> MVALSLKISIGNVVKTMQFEPSTMVYDACRMIRERIPEALAGPPNDFGLFLSDDDPKKGIWLEAGKALDYYMLRNGDTMEYRKKQRPLKIRMLDGTVKTIMVDDSKTVTDMLMTICARIGITNHDEYSLVRE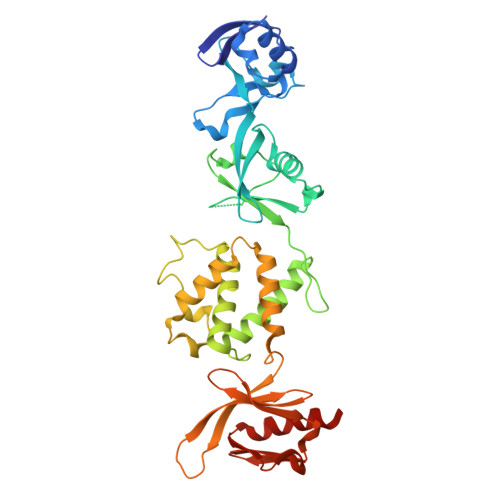LMEEKKDDELNWLDHGRTLREQGVEEHETLLLRRKFFYSDQNVDSRDPVQLNLLYVQARDDILNGSHPVSFDKACEFAGFQCQIQFGPHNEQKHKAGFLDLKDFLPKEYVKQKGERKIFQAHKNCGQMSEIEAKVRYVKLARSLKTYGVSFFLVKEKMKGKNKLVPRLLGITKECVMRVDEKTKEVIQEWSLTNIKRWAASPKSFTLDFGDYQDGYYSVQTTEGEQIAQLIAGYIDIIL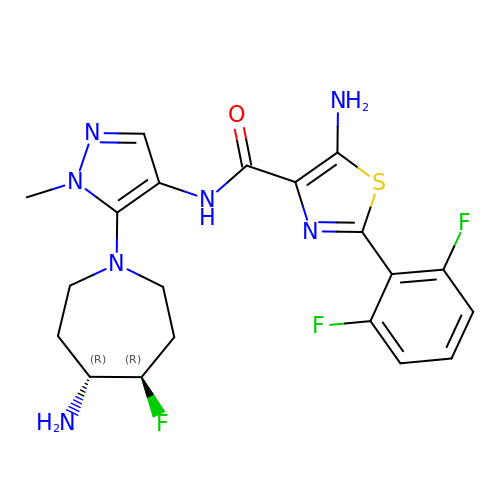5-amino-N-{5-[(4R,5R)-4-amino-5-fluoroazepan-1-yl]-1-methyl-1H-pyrazol-4-yl}-2-(2,6-difluorophenyl)-1,3-thiazole-4-carboxamide | C20 H22 F3 N7 O S | NHXVGMQFCYBLTL-ZWNOBZJWSA-N>[2x]MGSSHHHHHHSQDPMTVTANQVLRPRGPQIERLTDNRAKVVIEPLERGYGHTLGNALRRVLLSSIPGFAITEVEIDGVLHEYTTVEGLQEDVLDVLLNLKDVAIRMHSGDSATLSLSKQGPGTVTAADIRTDHNVEIINGDHVICHLTKDTALNMRLKIERGFGYQPAAARRRPDEETRTIGRLMLDASFSPVRRVAYAVEAARVEQRTDLDKLVIDIETNGTIDAEEAVRTAADILSDQLSVFGDFTHRDRGAAKPAASGVDPVLLRPIDDLELTVRSANCLKAESIYYIGDLIQKTEVELLKTPNLGKKSLTEIKEVLAQRGLALGMKLENWPPAGVAQHGMLG;> MTSYS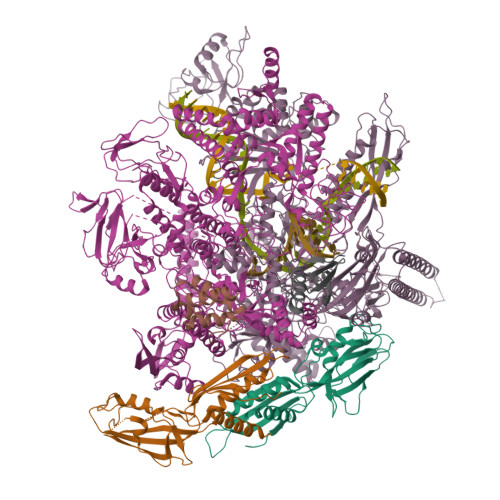FTEKKRIRKDFGKQRSILEVPFLLAIQVDSYREFLQEDVESTKRKDLGLHAALKSVFPISSYSGNAALEYVGYKLGQPVFDERECRQRGMSYGAPLRVTVRLVIYDRESSTKAIKYVKEQEVYLGEIPLMTGNGTFIVNGTERVIVSQLHRSPGVFFDHDRGKTHSSGKLLYSARIIPYRGSWLDFEFDPKDALFTRIDRRRKLPVSILLRALGYNNEEMLAEFFEINTFHINPDEGVQLELVPERLRGETLNFDLADGDKVIVEAGKRITARHVKQLEAAGVAALAVPDDYLVGRILSHDVVDGSTGELLANANDEISEDQLTAFRKAGVDAVGTLWVNDLDRGPYLSNTLRIDPTKTQLEALVEIYRMMRPGEPPTKEAAQNLFHNLFFTFERYDLSTVGRMKFNRRVGRKDVLGESVLYDKKYFAERNDEESKRLVAEHTDTSDILEVIKVLTEIRNGRGVVDDIDHLGNRRVRSVGEMAENVFRVGLVRVERAVKERLSMAESEGLTPQELINAKPVAAAIKEFFGSSQLSQFMDQNNPLSEVTHKRRVSALGPGGLTRERAGFEVRDVHPTHYGRVCTIETPEGPNIGLINSLAVFARTNQYGFLETPYRKVLDGKVSDDVEYLSAIEENEYVIAQANALTDAKNMLTEQFVPCRFQGESLLKPPSEVHFMDVSPMQTVSVAAALVPFLEHDDANRALMGANMQRQAVPTLRSQKPLVGTGIERAVARDSGVTVNALRGGVIEQIDAARIVVKVNEAEIGGGTDAGVDIYNLIKYTRSNQNTCINQRPLVNVGDVIARGDVLADGPSTDIGELALGQNMLIAFMPWNGYNFEDSILLSERVVEEDRYTTIHIEELTCVARDTKLGPEEISADIPNVSEQALNRLDESGVVYIGAEVRAGDIMVGKVTPKGESQLTPEEKLLRAIFGEKASDVKDSSLRVPPGMDGTVIDVQVFTRDGIEKDKRARQIEENEIKRVKKDFDDQFRILEAAIYARLRSQIVGKVANGGANLKKGDSVTDAYLDGLKKSDWFQLRMKDEDAADAIERAQKQIQAHEKEFEARFADKRGKITQGDDLAPGVLKMVKVFLAVKRRIQPGDKMAGRHGNKGVVSNVVPVEDMPYMATGESVDIVLNPLGVPSRMNIGQILEVHLGWAAKGLGRKIQRMLEAQAAVSELRKFLDDIYNHDNAINAQRVDLSQFSDEELLNLGKNLIDGVPMATPVFDGASEAEIKRMLELADLPQSGQTQLYDGRTGEAFDRKTTVGYMHYLKLNHLVDDKMHARSTGPYSLVTQQPLGGKAQFGGQRFGEMEVWALEAYGAAYTLQEMLTVKSDDVQGRNQMYKNIVDGEHEMVAGMPESFNVLVKEIRSLAIHMELEE;> MKDLLNLFNQQRQTLDFDAIKIALASPDLIRSWSYGEVKKPETINYRTFKPERDGLFCAAIFGPIKDYECLCGKYKRMKHRGVVCEKCGTEVTLAKVRRERMGHIDLASPVAHIWFLKSLPSRIGLMLDMTLRDIERVLYFEAYVVTEPGLTPLERRQLLTEEQYLTARQEYNDDFDAAMGAEAVYELLRTIDLQSEMTRLREEIASTGSETKLKRLTKRIKLIEAFLESGNRPEWMVMTVLPVLPPDLRPLVPLDGGRFATSDLNDLYRRVINRNNRLRRLLELNAPDIIVRNEKRMLQESVDALLDNGRRGRAITGTNKRPLKSLADMIKGKQGRFRQNLLGKRVDYSGRSVITVGPYLKLHQCGLPKKMALELFKPFVFAKLQRRGLATTIKAAKKLVEREEAEVWDILEEVIREHPVLLNRAPTLHRLGIQAFEPVLIEGKAIQLHPLVCTAFNADFDGDQMAVHVPLSLEAQLEARALMMSTNNILSPANGEPIIVPSQDVVLGLYYMSRALENKKGEGMVFANTSEVKRAYDNRVVELHAKVKVRITQVDVDAVDGKRTSGTSIVDTTVGRALLSEILPEGLPFQLANTEMTKKNISRLINSSYRLLGLKDTVVFADKLMYTGYAYATRAGVSIGIDDMLIPDEKKGILTEAEAEVLEIQEQYQSGLVTAGERYNKVVDIWSRTSERIAKAMMDTIGTEKVENAKGETIDQKSMNSLYIMADSGARGSQAQIRQLAGMRGLMARPDGSIIETPIKANFREGLNVQEYFNSTHGARKGLADTALKTANSGYLTRRLVDVAQDVVITEIDCGTTEGLIMTPIVEGGDVVEPLKERVLGRVVAEDVYLPGNDEEPIVTRNTLLDEAWVAKLEDASVQSVKVRSTISCESSFGVCARCYGRDLARGHQVNIGEAVGVIAAQSIGEPGTQLTMRTFHIGGAASRAAAVDNITVKTTGSVKFNNLKSVAHASGSLVAVSRSGELSVLDGHGRERERYKLPYGATITAKDGDAVKAGQSVANWDPHNHPIVSEVAGFIRFIDFVDGVTVIEKTDELTGLASREITDPKRRGAHAKELRPIVRIVDGKGNDLTIPNTDLPAQYLLPPRSIVNLQDGAAVGVGDVVAKIPQEASKTRDITGGLPRVADLFEARKPKDPAILAERSGIISFGKDTKGKQRLIIKDTDGSEHEELIPKYRQIIVFEGEHVTKGETVVDGEPSPQDILRLLGVEPLAAYLVKEIQDVYRLQGVKINDKHIEVITRQMLRKVEIVDQGNSKFLNGEQVERQRVIEENARLVKRNELPAKYDPVLLGITKASLATESFISAASFQETTRVLTEAAVRGTRDNLRGLKENVIVGRLIPAGTGLAYHAGRRKASGLTDSEMETLSGKPAGAEPVAALADAGADEE;> MARITVEDCLEVVNNRFELVMMASKRARQLANGVQPLIENAAASDKPTVMALREIAARRIDNALIDEVEKAERERAEREALEWAAAEVVADEDMSKNDD;> GAMAMNEFTQISGYVNAFGSQRGSVLTVKVENDEGWTLVEEDFDRADYGSDPEFVAEVSSYLKRNGGIKDLTKVLTR> DVSFRLSGATSSSYGVFISNLRKALPNERKLYDIPLLRSSLPGSQRYALIHLTNYADETISVAI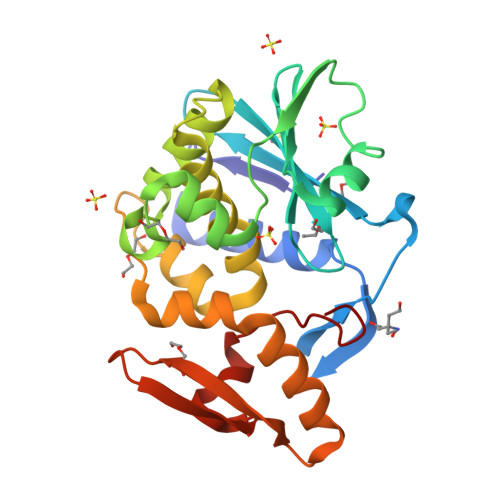DVTNVYIMGYRAGDTSYFFNEASATEAAKYVFKDAMRKVTLPYSGNYERLQTAAGKIRENIPLGLPALDSAITTLFYYNANSAASALMVLIQSTSEAARYKFIEQQIGKRVDKTFLPSLAIISLENSWSALSKQIQIASTNNGQFESPVVLINAQNQRVTITNVDAGKVTSDIALLLNRNNMA> MSSFKYKNSAAGASMQSAANITLRQILEPNNVNLRSKKTHIVCTLGPACKSVETL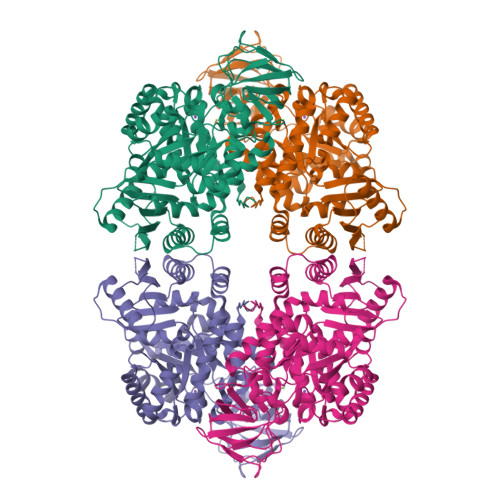VKLIDAGMDICRFNFSHGSHEDHKEMFNNVLKAQELRPNCLLGMLLDTKGPEIRTGFLKNKEVHLKEGSKLKLVTDYEFLGDETCIACSYKKLPQSVKPGNIILIADGSVSCKVLETHEDHVITEVLNSAVIGERKNMNLPNVKVDLPIISEKDKNDILNFAIPMGCNFIAASFIQSADDVRLIRNLLGPRGRHIKIIPKIENIEGIIHFDKILAESDGIMIARGDLGMEISPEKVFLAQKLMISKCNLQGKPIITATQMLESMTKNPRPTRAEVTDVANAVLDGTDAVMLSGETAGGKFPVEAVTIMSKICLEAEACIDYKLLYQSLVNAIETPISVQEAVARSAVETAESIQASLIIALTETGYTARLIAKYKPSCTILALSASDSTVKCLNVHRGVTCIKVGSFQGTDIVIRNAIEIAKQRNMAKVGDSVIAIHGIKEEVSGGTNLMKVVQIELEHHHHHH> AFEDELGAQPPLGFFDPLGLVADGD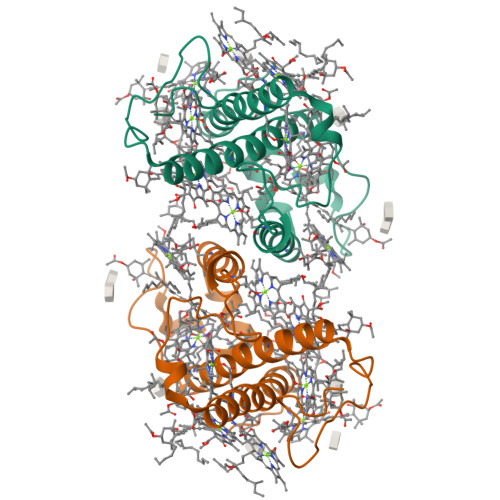QEKFDRLRYVEIKHGRISMLAVVGYLVQEAGVRLPGTIDYSGKTFAEIPNGFAAFKEIPAGGLVQLLFFIGVLESSVMRDLTGEAEFVGDFRNGAIDFGWDTFDEETQFKKRAIELNQGRAAQMGILALMVHEQLGVSLLPQ>MELIRIAMKKDLENDNSLMNKWATVAGLKNPNPLYDFLNHDGKTFNEFSSIVNIVKSQYPDREYELMKDYCLNLDVKTKAARSALEYADANMFFEIEDALIDSMISCSNMKSKEYGKVYKIHRELSKGEIDVFEASANIGKQRIKTAEMNIFSKMLLMYDCLNKGNFAPMMLLFQQIDLSEIKENRYLKNSFETRINVLLSNIYLNENNLELCREYAQKAISSTDTQRFLVFSYLTIGTSYIFSDFNLSKQNYLIGLKFAKGNPGFEEFFKRNLSFLNNFWNKENEWINYDSDAVTDMQEVIFELINHKELSKALQLLNKLEERDQNENELGFHYYLKGLITNEKEAFFKSVEY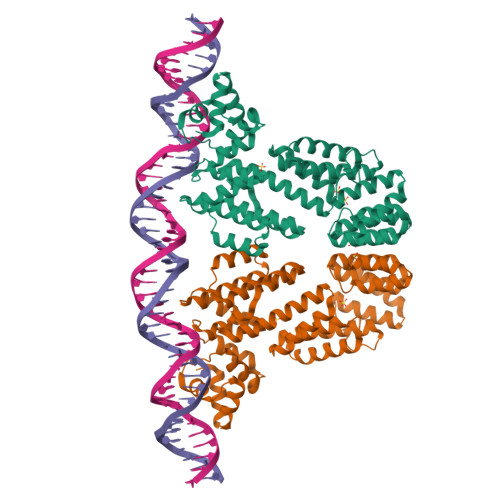FKASQDKLSIKMPLIQLEKMGENPRLLKIITM[2x]{(E)-(3R,6S,9R)-3-[(1S,3R)-3-((S)-1 -BUTYLCARBAMOYL-2-METHYL-PROPYLCARB AMOYL)-1-HYDROXY-BUTYL]-6-METHYL-5, 8-DIOXO-1,11-DITHIA-4,7-DIAZA-CYCLO PENTADEC-13-EN-9-YL}-CARBAMIC ACID TERT-BUTYL ESTER | C31 H55 N5 O7 S2 | 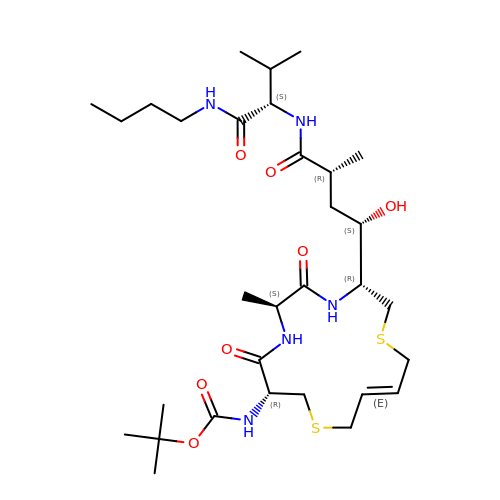YFVXRNZNJJXEKV-DYASFXQMSA-N>[3x]MDNKLGLNKMNKTLIALAVSAAAVATGAYADGINQSGDKAGSTVYSAKGTSLEVGGRAEARLSLKDGKAQDNSRVRLNFLGKAEINDSLYGVGFYEGEFTTNDQGKNASNNSLDNRYTYAGIGGTYGEVTYGKNDGALGVITDFTDIMSYHGNTAAEKIAVADRVDNMLAYKGQFGDLGVKASYRFADRNAVDAMGNVVTETNAAKYSDNGEDGYSLSAIYTFGDTGFNVGAGYADQDDQNEYMLAASYRMENLYFAGLFTDGELAKDVDYTGYELAAGYKLGQAAFTATYNNAETAKETSADNFAIDATYYFKPNFRSYISYQFNLLDSDKVGKVASEDELAIGLRYDFHHHHHH

OmpU is a major OMP that constitutes about 30% of the total outer membrane protein when V. cholerae is grown in a medium containing 1% NaCl and nearly 60% when it is grown in salt-free medium. It is characterized as a porin that forms non­specific β-barrel channels allowing free diffusion of hydrophilic molecules across the OM. Apart from its porin function, OmpU has also been shown to confer the pathogen with resistance to bile and antibacterial peptides. OmpU has long been proposed as a potential virulence factor involved in pathogen–host interactions during infection, being capable of making physical contact with and adhering to host cells, as well as triggering subsequent invasion by the pathogen.

Here, we present the first crystal structure of the V. cholerae OmpU trimer, at a resolution of 2.2 Å. In addition to the ordered water molecules, 13 detergent molecules and six glycerol compounds were manually assigned. Loop L3 deviates from the wall of the barrel and extends into the barrel to serve as a constriction loop in the pore lumen. As in all other bacterial porins, the β-barrel surrounds an aqueous pore through which cargoes are diffused. A unique structural feature of OmpU is the presence of an extended N-terminal coil (Gly32–Ser42) in the pore lumen in addition to the conventional localization of the constriction loop L3 within the channel, which is unprecedented in solved structures of bacterial porins to the best of our knowledge. OmpU possesses a unique N-terminal coil consisting of Gly32–Ser42 that extends into the pore at the periplasmic side and forms a second gate with the constriction loop L3. Remarkably, L4 is the longest loop on the extracellular side and, instead of being a single long loop, it contains two short antiparallel β-sheets that resemble a β-hairpin structural motif but are connected by a loop containing more than five residues. Although L4 of OmpU is shorter than L4 of OmpK36, L4 of OmpU protrudes further into the extracellular space and projects over L1 of the adjacent protomer to the proximity of L8. The graph shows that the minimum radius in native OmpU is ∼3.1 Å, which is slightly smaller than the value of 3.2 Å found in OmpU with a deleted N-terminus.> MKEEATTLPQQFIKKYRLLLGEEASDFFSALEQGSVKKGFRWNPLKPAGLDMVQTYHSEELQPAPYSNEGFLGTVNGKSFLHQAGYEYSQEPSAMIVGTAAAAKPGEKVLDLCAAPGGKSTQLAAQMKGKGLLVTNEIFPKRAKILSENIERWGVSNAIVTNHAPAELVPHFSGFFDRIVVDAPCSGEGMFRKDPNAIKEWTEESPLYCQKR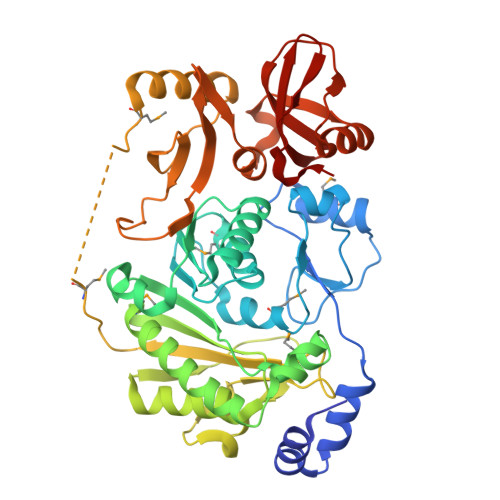QQEILSSAIKMLKNKGQLIYSTCTFAPEENEEIISWLVENYPVTIEEIPLTQSVSSGRSEWGSVAGLEKTIRIWPHKDQGEGHFVAKLTFHGQNQMHKEKKTRKKSKVQMTKEQEKLWTEFSNDFHYEATGRLLVFNDHLWEVPELAPSLDGLKVVRTGLHLGDFKKNRFEPSYALALATKKIENIPCLPITQKEWQSYTAGETFQRDGNQGWVLLVLDKIPVGFGKQVKGTVKNFFPKGLRFH>[2x]MKKHHHHHHMTELRDETPLFHKGEI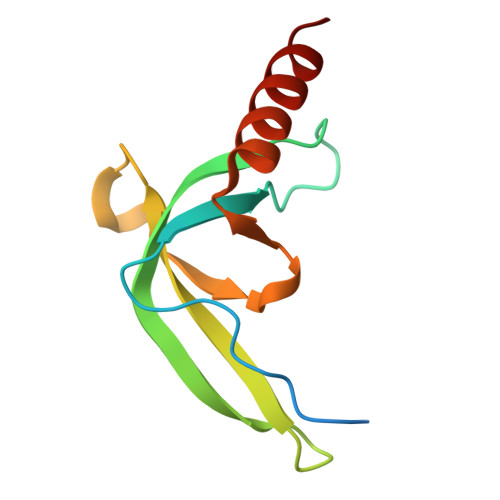VLCYEPDKSKARVLYTSKVLNVFERRNEHGLRFYEYKIHFQGWRPSYDRAVRATVLLKDTEENRQLQRELAEAAKL>GAMGIEIGENVLLEYIEENELKKAKSKAVSIENNELLIAYPVDVVTGRTVILHNDMEVTVEFVGKDEVPYRFISRIKGKVKDKLQMICLEMPPREKMKRIQRRQYVRTDAVLDVQIQPGNEEEIRTLSYNISAGG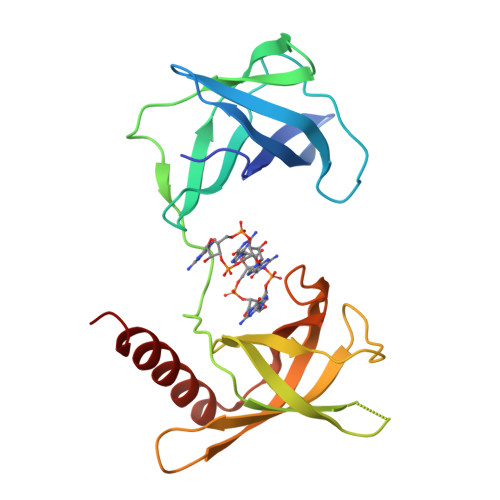IAVVLADGLSFQSGESLRLIIRLPEEEHTRQIETEAVVRRIFNDPKSEKRKMTLEYSEIAAGDQQALLQYCIRRQLNKRRK[2x]In group B rotavirus, which causes significant diarrheal outbreaks in adults, the VP8* domain (VP8*B) surprisingly lacks sequence similarity with VP8* of group A or group C rotavirus. Here, by using the recently developed AlphaFold2 for ab initio structure prediction and validating the predicted model by determining a 1.3-Å crystal structure, we show that VP8*B exhibits a novel fold distinct from the galectin fold. This fold with a β-sheet clasping an α-helix represents a new fold for glycan recognition based on glycan array screening, which shows that VP8*B recognizes glycans containing N-acetyllactosamine moiety. Despite the novel fold, based on our glycan screening study, it is likely that VP8*B, similar to the VP8* of RVA and RVC, retains the same functionality of mediating the initial cell attachment by recognizing specific glycans in the gut.

As a representative VP8*B, the amino acid sequence of a human RVB, isolated from a gastroenteritis outbreak in India32, was expressed and purified for structure determination by X-ray crystallography. We used the well-ordered region of VP8*B (residues 83–192) in the AlphaFold2-predicted fold as a search model for MR, and determined the crystal structure of native VP8*B at 1.3-Å resolution. The crystallographic asymmetric unit contains two VP8*B molecules in addition to a short peptide. Although we purified and crystallized the recombinant VP8*B containing residues 65–233 of VP4, only the residues F78-N202 are observed in the crystal structure. The electron density of the N- and C-terminal residues are not observed due to their flexibility or a proteolytic cleavage that may have occurred during crystallization. The small peptide with four residues could be the protease cleavage product co-crystallized with the globular portion of the VP8*B. The electron density of the side chains does not match any residues of the N or C terminus of VP8*B, possibly due to heterogeneity of the short peptide and the lack of sequence specificity of the peptide-binding. The VP8*B structure contains seven β-strands and one α-helix. Five of these β-strands form a twisted antiparallel β-sheet that surrounds a central α-helix. Structural comparison of the two shows a high degree of similarity between the models with a Cα RMSD of 0.398 Å and 0.403 Å with the two VP8*B molecules in the asymmetric unit, respectively. Interestingly, the side chain of Q195 also interacts with His131 that is present in different conformations in the predicted and experimental models, suggesting that subtle changes in solution may affect glycan-binding during virus infection.

>[2x]MSLGQSDLHIDPTQFIMYSGTISNGISYVNQAPSCGTVLSLKFTPGNSSLIENLHIEPYKVEVLKIEHVGDVSRATLLSDIVSLSTAQKKLLLYGFTQPGVQGLTGDVVSVETKRIPTPTQTNLLTIEDSIQCFTWDMNCANARSTNQDSRLIIYEQEDGRSHHHHHH;> GAAG>MSLIVSTIASHSSLQILLGAKKEGFKTRLYVSPKRRPFYSSLPI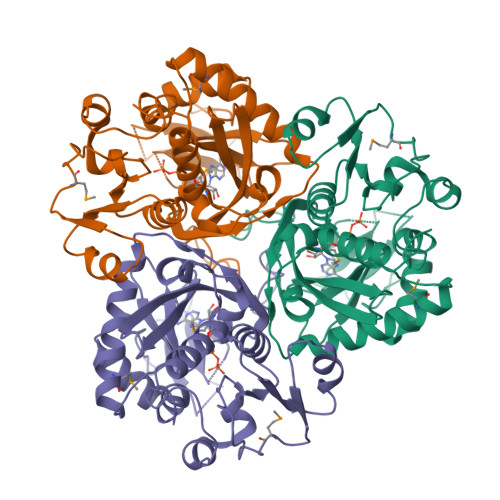VDDLVVAEEMTSILNDDGIVVPHGSFVAYLGIEAIEKAKARFFGNRRFLKWETTFELQDKALEGAGIPRVEVVEPEDAKPDELYFVRIEGPRGGSGHFIVEGSELEERLSTLEEPYRVERFIPGVYLYVHFFYSPILERLELLGVDERVLIADGNARWPVKPLPYTIVGNRAIALRESLLPQLYDYGLAFVRTMRELEPPGVIGPFALHFAYDGSFKAIGIASRIDGGSNADHWYSELYWGERLSMGRRIARELRLAEEEDRLEEVVTEGHHHHHH[3x]>GPSQELTNEKEKALQAQVQYQQQHEQQKKDLEILHQQNIHQLQNRMSELEAANKDLTERKYKGDSTIRELKAKLSGVEEELQRT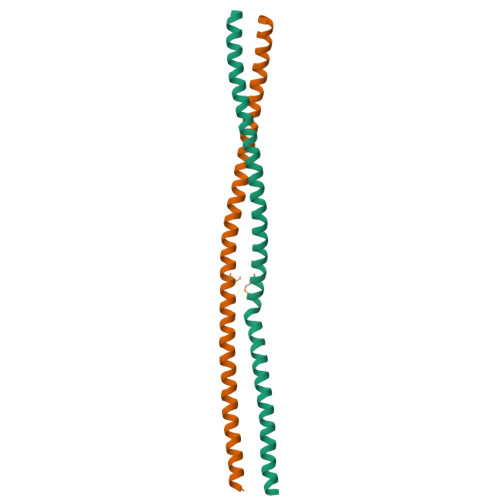KQEVLSLRRENSTLDVECHE[6x]>TQVFDLEGYGAISRAMGGTSSSYYTGNAALISNPATLSFA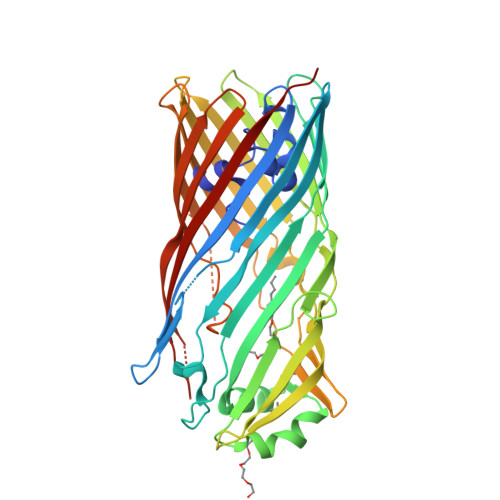PDGNQFELGLDVVTTDIKVHDSHGAEAKSSTRSNNRGPYVGPQLSYVAQLDDWRFGAGLFVSSGLGTEYGSKSFLSQTENGIQTSFDNSSRLIVLRAPIGFSYQATSKLTFGASVDLVWTSLNLELLLPSSQVGALTAQGNLSGGLVPSLAGFVGTGGAAHFSLSRNSTAGGAVDAVGWGGRLGLTYKLTDNTVLGAMYNFKTSVGDLEGKATLSAISGDGAVLPLDGDIRVKNFEMPASLTLGLAHQFNERWVVAADIKRAYWGDVMDSMNVAFISQLGGIDVALPHRYQDITVASIGTAYKYNNDLTLRAGYSYAQQALDSELILPVIPAYLKRHVTFGGEYDFDKDSRINLAISFGLRERVQTPSYLAGTEMLRQSHSQINAVVSYSKNFHHHHHH[2x]> GIPTLYTPGSGQFLTTDDFQTPCMLPKFQPTPVIDIPGEVKNFLEVVQVESLVEINNVESAEGVAR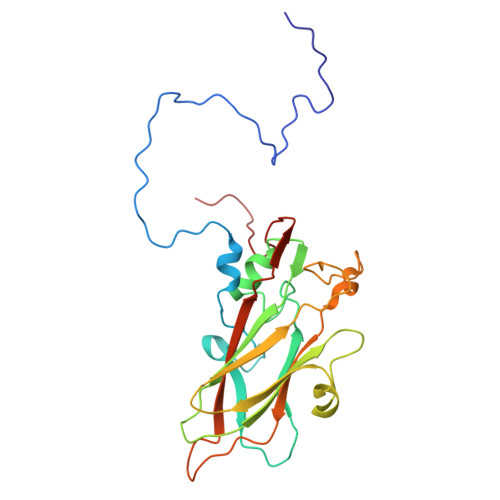YRIPLNVQDAMDGQIMALRVDPGIDGPMQSTLLGVFTRYYAQWSGSLDFTFMFCGTFMTTGKVIIAYTPPGGDQPTNRRQAMLGTHVVWDFGLQSSITLVVPWISSGHFRGTTLENTIYKYRYYEAGYITMWYQTNMVVPPNFPTTASILMFVAAQPNFSLRILKDRPDISQEGALQ>PEFLNNTEPLCNVSGFAIVSKDNGIRIGSRGHVFVIREPFVACGPTECRTFFLTQGALLNDKHSNNTVKDRSPYRALMSVPLGSSPNAYQAKFESVAWSATACHDGKKWLAVGISGADDDAYAVIHYGGMPTDVVRSWRKQILRTQESSCVCMNGNCYWVMTDGPANSQASYKIFKSHEGMVTNEREVSFQGGHIEECSCYPNLGKVECVCRDNWNGMNRPILIFDEDLDYEVGYLCAGIPTDTPRVQDSSFTGSCTNAVGG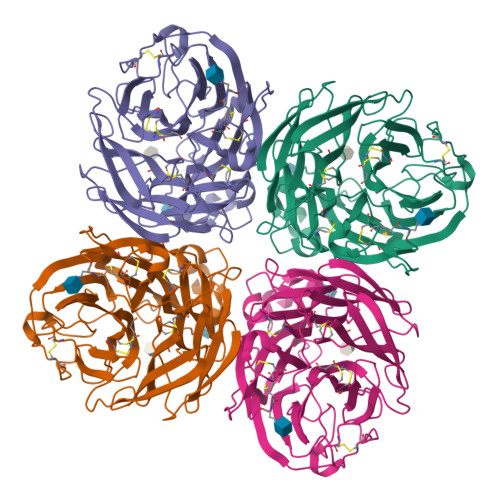SGTNNYGVKGFGFRQGNSVWAGRTVSISSRSGFEILLIEDGWIRTSKTIVKKVEVLNNKNWSGYSGAFTIPITMTSKQCLVPCFWLEMIRGKPEERTSIWTSSSSTVFCGVSSEVPGWSWDDGAILPFDIDKM[2x]(3R,5R)-7-{3-[(4-carbamoylphenyl)sulfamoyl]-4,5-bis(4-fluorophenyl)-2-(1-methylethyl)-1H-pyrrol-1-yl}-3,5-dihydroxyheptanoic acid | C33 H35 F2 N3 O7 S | 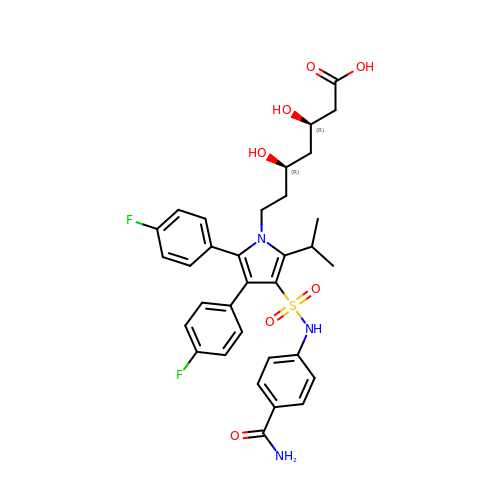IYYNBGFAAGBIAX-KAYWLYCHSA-N> MRGSHHHHHHGSLQVTVRDAINQGMDEELERDEKVFLLGEEVAQYDGAYKVSRGLWKKYGDKRIIDTPISEMGFAGIAVGAAMAGLRPICEFMTFNFSMQAIDQVINSAAKTYYMSGGLQPVPIVFRGPNGASAGVAAQHSQCFAAWYGHCPGLKVVSPWNSEDAKGLIKSAIRDNNPVVVLENELMYGVPFEFPPEAQSKDFLIPIGKAKIERQGTHITVVSHSRPVGHCLEAAAVLSKEGVECEVINMRTIRPMDMETIEASVMKTNHLVTVEGGWPQFGVGAEICARIMEGPAFNFLDAPAVRVTGADVPMPYAKILEDNSIPQVKD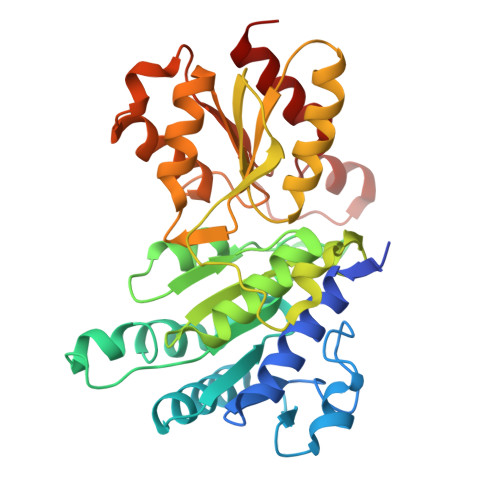IIFAIKKTLNI>MSPTAFPAAETATAPATAVDPGPELDGGDFALPEGGLDDDRRLRALDAVDEYLTRKRKHLVGYQATQDMQGT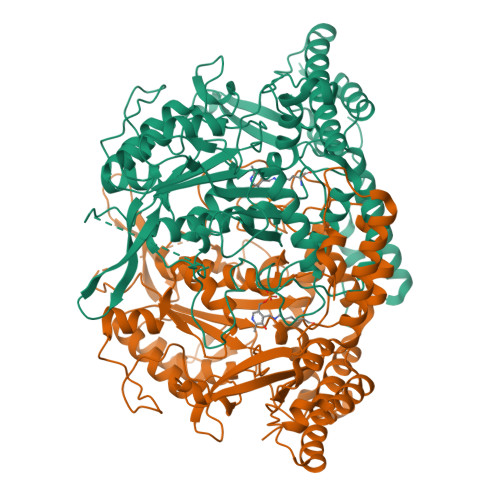ALDLARFMPNNINNLGDPFQSGGYKPNTKVVERAVLDYYAKLWHAERPHDPADPESYWGYMLSMGSTEGNMYALWNARDYLSGKALIQPPTAPFDAVRYVKADPDRRNPNAHHPVAFYSEDTHYSFAKAVAVLGVETFHAVGLEKYADECPLVDPVTGLRTWPTEVPSRPGPSGLSWDGPGEIDVDALAVLVEFFAAKGHPVFVNLNLGSTFKGAHDDVRAVCERLLPIFERHGLVQREVVYGSCPQTGRPLVDVRRGFWIHVDGALGAGYAPFLRLAAEDPEGYGWTPEAELPEFDFGLRLPTAGHGEVDMVSSIAMSGHKWAGAPWPCGIYMTKVKYQISPPSQPDYIGAPDTTFAGSRNGFSPLILWDHLSRYSYRDQVERIREAQELAAYLERRLTAMERELGVELWPARTPGAVTVRFRKPSAELVAKWSLSSQDVLMVPGDETTRRSYVHVFVMPSVDRAKLDALLAELAEDPVILGAP[2x]>[6x]MAHHHHHHMSNERTFIALKPDAVQRGLVGTIIARFEQKGFKLVALKLITP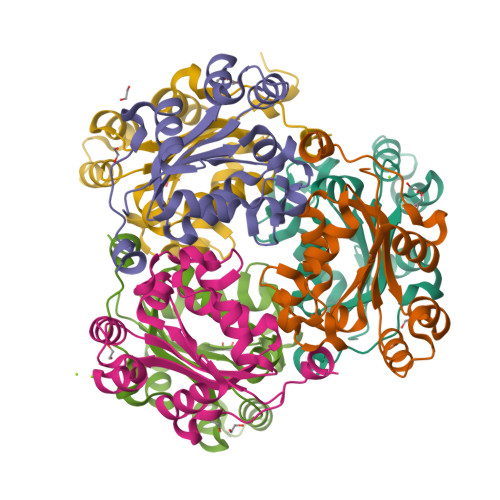SADLAKKHYAEHDGKPFFNGLVEFLTSGPVAAMVWEGKGVVAAARKMIGATKPLESAPGTIRGDFAIDVGRNIIHGSDAVETAQREIALWFQDSELNEWTPTQNKWIYE> XMLRRNPTAIQITAEDVLAYDEEKLRQTLDSESTTEEALQKNEESTRLSPEKKKIIR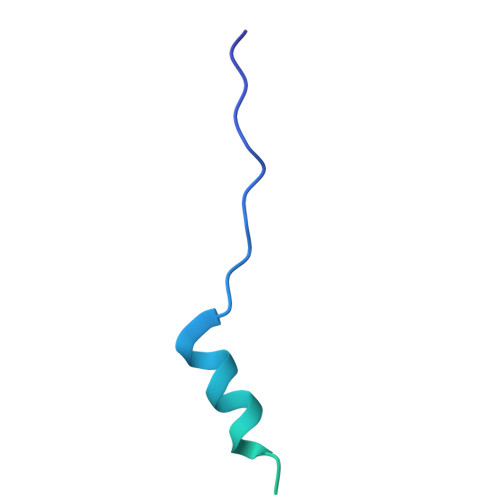ERRIGITQIFDSSMHPSQGGAAQS>[2x]GSHMEDITSGLKQLDSTYKETNQQVLKNLDEIFST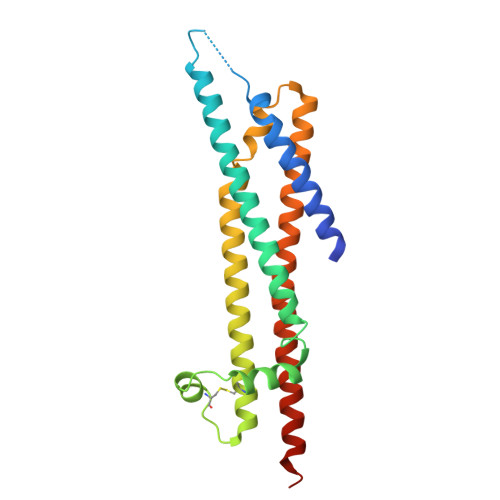TSPSANDKIGKEDALNIKKAAIALRGDLALLKANFEANELFFISEDVIFKTYMSSPELLLTYMKINPLDQKTAEQQCGISDKVLVLYCEGKLKIEQEKQNIRERLETSLKAYQSNIGGTASLITASQTLVESLKNKNFIKGIRKLMLAHDKVFLNYLEKLDALEISLEQSKRQYLQERQSSKVIVK[(2R)-2-{2-[hydroxy(methyl)amino]-2-oxoethyl}-5-(3-methoxyphenyl)pentyl]phosphonic 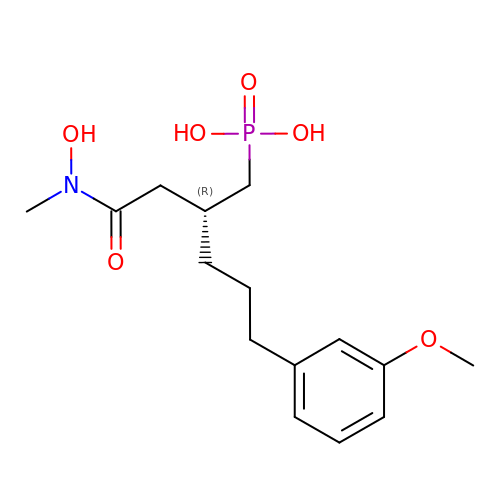acid | C15 H24 N O6 P | OCDQDBAFBVPPGL-CYBMUJFWSA-N(1S)-1,5-anhydro-1-(3-chloro-2-hydroxy-5-methoxyphenyl)-D-glucitol | C13 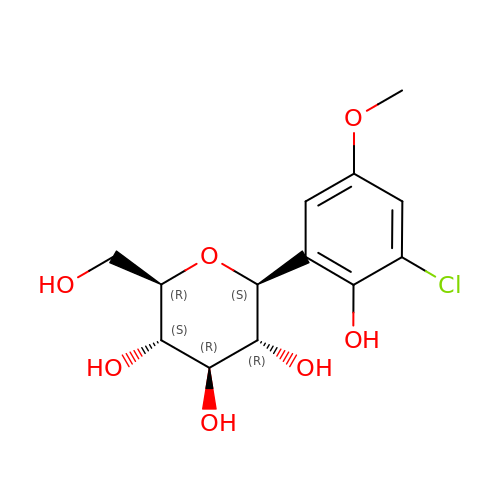H17 Cl O7 | MBLREHINSXJTTD-ZMHPAJMFSA-N[1-fluoro-2-(imidazo[1,2-a]pyridin-3-yl)ethane-1,1-diyl]bis(phosphonic acid) | C9 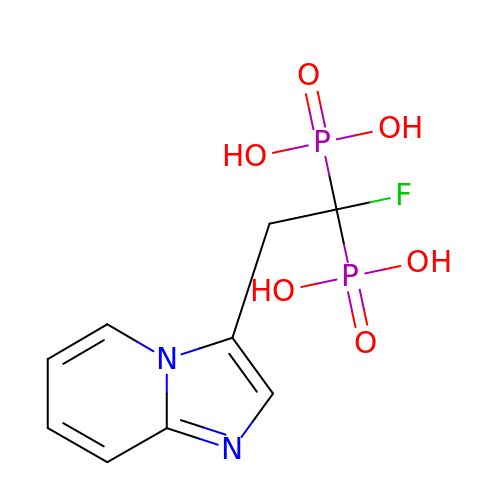H11 F N2 O6 P2 | MGBVLKIPHVCMLV-UHFFFAOYSA-N>[4x]LVSRAAIAATAMASLLLLIKIFAWWYTGSVSILAALVDSLVDIGASLTNLLVVRYSLQPADDNHSFGHGKAESLAALAQSMFISGSALF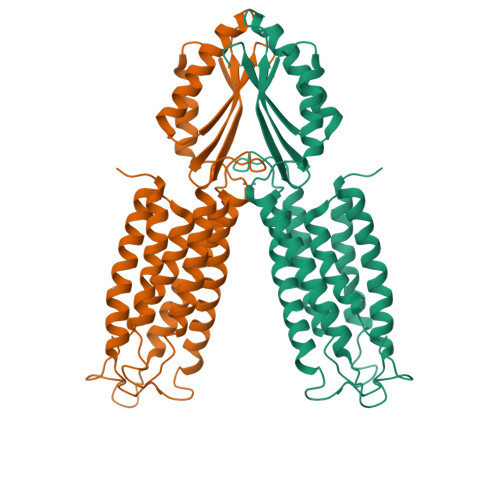LFLTGIQHLISPTPMTDPGVGVIVTIVALICTIILVSFQRWVVRRTQSQAVRADMLHYQSDVMMNGAILLALGLSWYGWHRADALFALGIGIYILYSALRMGYEAVQSLLDRALPDEERQEIIDIVTSWPGVSGAHDLRTRQSGPTRFIQIHLEMEDSLPLVQAHMVADQVEQAILRRFPGSDVIIHQDPCSVV> MIEAPDVKPWLFLIKPYEGESLSHFLGRFRRANHLSASGLGTLAGIGAIVARWERFHFNPRPSQQELEAIASVVEVDAQRLAQMLPPAGVGMQHEPIRLCGACYAESPCHRIEWQYKSVWKCDRHQLKILAKCPNCQAPFKMPALWEDGC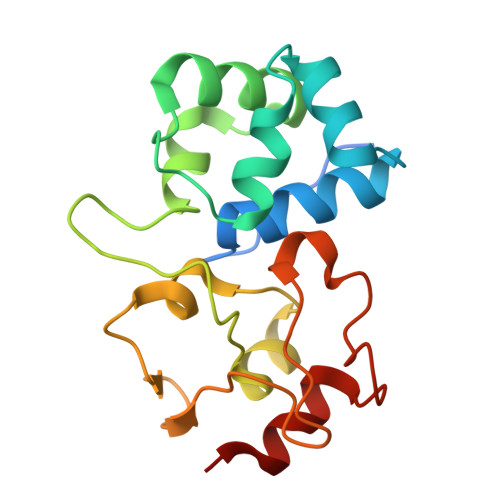CHRCRMPFAEMAKLQKV>MRIPLVGKDSIESKDIGFTLIHEHLRVFSEAVRQQWPHLYNEDEEFRNAVNEVKRAMQFGVKTIVDPTVMGLGRDIRFMEKVVKATGINLVAGTGIYIYIDLPFYFLNRSIDEIADLFIHDIKEGIQGTLNKAGFVKIAADEPGITKDVEKVIRAAAIANKETKVPIITHSNAHNNTGLEQQRILTEEGVDPGKILIGHLGDTDNIDYIK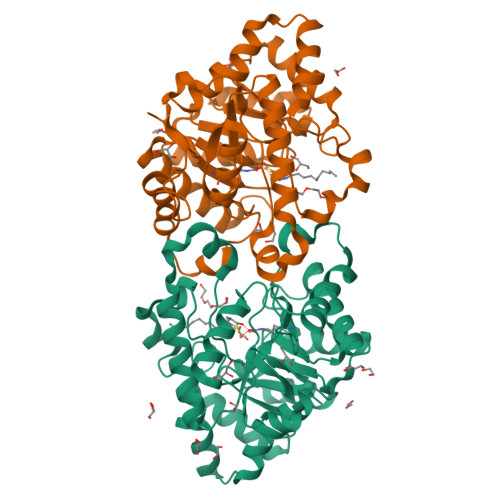KIADKGSFIGLDRYGLDLFLPVDKRNETTLRLIKDGYSDKIMISHDYCCTIDIGTAKPEYKPKLAPRWSITLIFEDTIPFLKRNGVNEEVIATIFKENPKKFFS[4x]>[4x]GAMGSSEAEIKVREATSNDPWG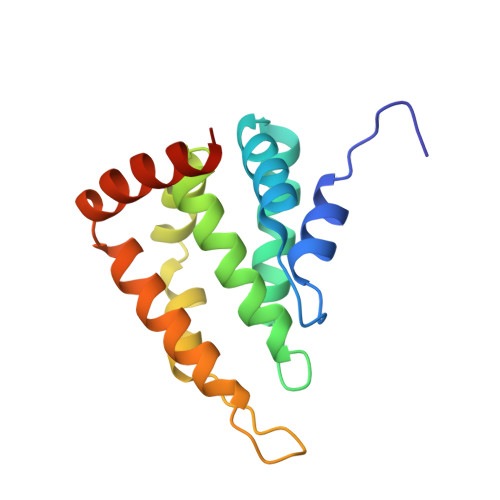PSSSLMSEIADLTYNVVAFSEIMSMVWKRLNDHGKNWRHVYKAMTLMEYLIKTGSERVAQQCRENIYAVQTLKDFQYIDRDGKDQGVNVREKAKQLVTLLKDEERLREERIHALKTKEKMAQT>STAFVDQDKQMANRLNLSPLERSKIEKQYGGATTLAFISNKQNELAQILSRADILKIASYDCAAHALQAVLDCGPMLGKRGFSQSDIVKIAGNIGGAQALQAVLDLESMLGKRGFSRDDIAKMAGNIGGAQTLQAVLDLESAFRERGFSQADIVKIAGNNGGAQALYSVLDVEPTLGKRGFSRADIVKIAGNTGGAQALHTVLDLEPALGKRGFSRIDIVKIAANNGGAQALHAVLDLGPTLRECGFSQATIAKIAGNIGGAQALQMVLDLGPALGKRGFSQATIAKIAGNIGGAQALQTVLDLEPALCERGFSQATIAKMAGNNGGAQALQTVLDLEPALRKRDFRQADIIKIAGNDGGAQALQAVIEHGPTLRQHGFNLADIVKMAGNIGGAQALQAVLDLKPVLDEHGFSQPDIVKMAGNIGGAQALQAVLSLGPALRERGFSQPDIVKIAGNTGGAQALQAVLDLELTLVEHGFSQPDIVRITGNRGGAQALQAVLALELTLRERGFSQPDIVKIAGNSGGAQALQAVLDLELTFRERGFSQADIVKI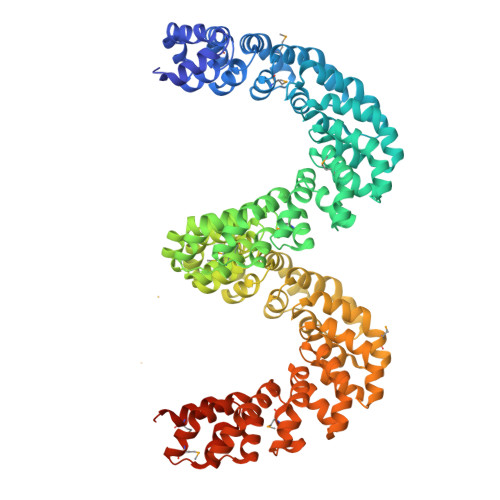AGNDGGTQALHAVLDLERMLGERGFSRADIVNVAGNNGGAQALKAVLEHEATLNERGFSRADIVKIAGNGGGAQALKAVLEHEATLDERGFSRADIVRIAGNGGGAQALKAVLEHGPTLNERGFNLTDIVEMAANSGGAQALKAVLEHGPTLRQRGLSLIDIVEIASNGGAQALKAVLKYGPVLMQAGRSNEEIVHVAARRGGAGRIRKMVAPLLERQGGSEFELENLYFQGELRRQASALE[2x]Members of the family of the Tri Longin domain (TLD) Rab-GEFs (guanine nucleotide exchange factors) act as activators of a subset of Rabs that play a critical role in late endosomal biogenesis. The best-studied TLD Rab-GEF is MC1, which activates Rab7 (Ypt7 in yeast) in endosomal maturation and autophagy. While GAPs promote the intrinsically low GTP hydrolysis rate of Rabs to switch them off, GEFs stimulate nucleotide release and the loading of Rab with GTP to convert the GTPase to its active conformation. To gain molecular insight into the targeting mechanism of MC1 and to understand how the complex is built in three dimensions, we determined the cryogenic electron microscopy (cryo-EM) structure of a stable MC1 complex from Chaetomium thermophilum.

We then produced an equivalently truncated complex CtMC1Δ (CtMon1 141 to 665, CtMon1ΔN; CtCcz1 1 to 796Δ361 to 460, CtCcz1ΔL), which expressed at an improved yield and also exhibited higher stability than the wild type. The orientation of the CtMC1Δ particles on the cryo-EM grids was tremendously improved in comparison to the wild type, allowing us to obtain a three-dimensional (3D) reconstruction of the complex with an average resolution of 3.85 Å. The quality of the map was sufficient to build an atomic model of ∼75% of CtMC1Δ, including all Longin domains of Mon1 and Ccz1. The three Longin domains (LDs) of both Mon1 and Ccz1 are triangularly arranged and form together the backbone of MC1, which has a pseudo twofold symmetry. Mon1 and Ccz1 interact via their LD1 and LD3 domains. The respective LDs (LD1-LD1 and LD3-LD3) share a large interface and form two continuous cross-subunit β-sheets. The two continuous β-sheets are a defining structural feature of MC1 that results in a two-layered complex architecture. Thus, structurally and functionally, the MC1 complex can be divided into a top “catalytic” layer and a base “localization” layer. An electrostatic surface potential map of CtMC1Δ reveals a large positively charged patch stretching over LD2 and LD3 of Mon1 and a negatively charged region on the surface of LD1 and LD3 of Ccz1. Taken together, we conclude that the basic patch formed by LD2/3 of Mon1 is responsible for binding to PIP lipids.

> TGTAGDLASLLAGDGLGRKSKAWRVLRAQQQACGEGSGEEGEITEIEGLGLGEGMEGFERELDNIPDTLPDDERLALWKGKLKHYLILSSAGKPIWSRHGDLSLVNSTMGVVQTIISFYEGARNPLLGFTAGKVRFVILIKGPLYFVAISRLRESDAQLRAQLEALYMQILSTLTLPILTNIFAHRPSTDLRGPLQGTESLLASLADSFTKGSPSTLLSALECLRLRKSQRQAITNIFLKSRCEELLYGLLVAGGKLVSVIRPRKHSLHPSDLQLIFNMLFESGGIKGNGGENWIPLCLPAFNNTGYLYMYVSFLDDKAPDDQNQPPESSNLDASNKNSSNTPDDDLTALILISPSREAFYALQSMRTRLVSQLLSTGYLSLIRSTALSGRPSITSILPKTPLLHFLYKSRPNVQWCMSSLSSLTPPGATATETLLARRKLMSVYEELHAALHARHAHLRVVYSTADEKEGEGLACLGWSTPAFEVYCVAPGCVGRAGMAREVNRVVQWARREEERLFILGGGVF;> MTTPVSPSPSGIIPAQLGFLAIYNPALGTTDETLEDQIVYYATASTLSQARRRHRRPRRRDRQRAQSVVKDSRPNAAGATGDSEAVAEDKDPVSKEERHERLRQIGLAQGMVEFAKSFSDGEPVDTIDTEKARVILVEVEEGWWILASIDLTRLPLPQIKTPTSSSAPPPAPNLNPLPPEPAYEYSSREVKPPSLLRADLLRAYDLFLLHHGSSLSSLLASQGRAQLVASLTRFWDHFLATWNVLLHGNPACDVFGGIKLAASGELGIGVGEEERGSGEREVLEGLVERVEGLVDVVVGRYGGPPSEKGPEEEQWLGLGGEVGEEDGAVFLGVGALDRKSLRGVVQWMEEVYVWGENAFGKPRRDLSTGHFLLGLSECSEEELTSSQANPKAIFVELKPSYQHPSRKIPPEDPQPLGKVGPELPRDHTARLRPVIYVSQPFIYILLFSEITPSPSTWPTLAESLHAQLSPLQKPLLHSTSYRPERPVVETTSSSGTTTQHQIFDLVYDTETLTLQSTIPNIPDPFPYSATTPTGHSTGQQHHQQSIWTRVEALQTHAQILAILSSGRAIPTDPSSFTHLPWEEGERTCKTARGWWIVWTRVVEHSPPDAVSLHHARDDDDNDDDASCSVLGHLRSVSSSHAAGSTSSSSGSGFGLGAIPGLGGLGGWAADGATRLAQGIGIDTRRYVEGLLTSLGR> MAQEGDFPMPFISAKSSPVIPLDGSVKIQCQAIREAYLTQLMIIKNSTYREIGRRLKFWNETDPEFVIDHMDANKAGRYQCQYRIGHYRFRYSDTLELVVTGLYGKPFLSADRGLVLMPGENISLTCSSAHIPFDRFSLAKEGELSLPQHQSGEHPANFSLGPVDLNVS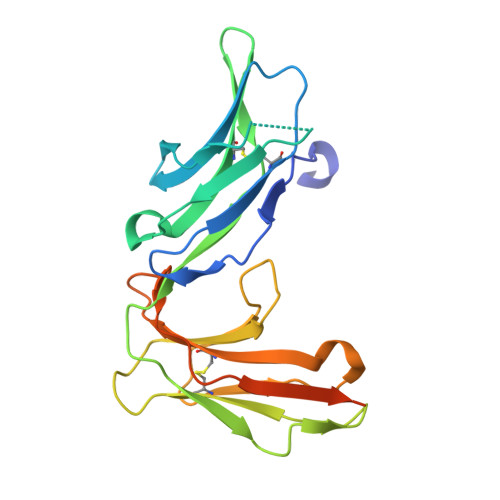GIYRCYGWYNRSPYLWSFPSNALELVVTDSIHQDYTTQNLILEHHHHHH> MGSDKIHHHHHHMQPFRVTLVEDEPSHATLIQYHLNQLGAEVTVHPSGSAFFQHRSQLSTCDLLIVSDQLVDLSIFSLLDIVKEQTKQPSVLILTTGRHELIESSEHNLSYLQKP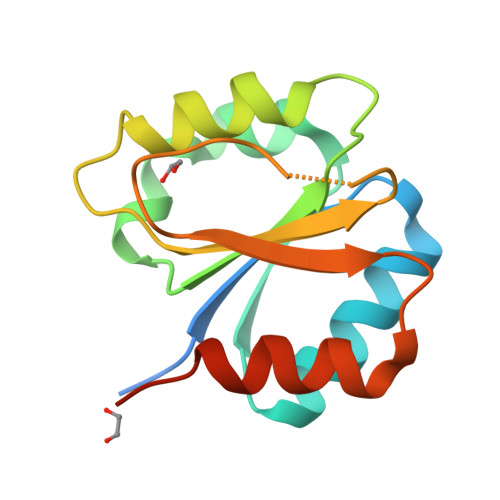FAISELRAAIDYHKPSMGVTMNV[[(1R,3S,5S)-3-(2-azanyl-6-oxidanylidene-3H-purin-9-yl)-2-methylidene-5-oxidanyl-cyclopentyl]methoxy-oxidanyl-phosphoryl] 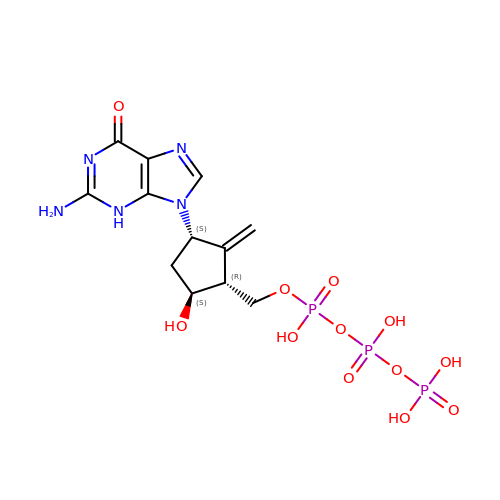phosphono hydrogen phosphate | C12 H18 N5 O12 P3 | YMBBDUCQYPKKJK-FXQIFTODSA-N>[2x]ATAQMQPDFWANQQAQFANEQNRLEQERVQQLQQQQAQQELFQQQLQKAQQDMMNMQLQQQNQHQNDLIALTNQYEKDQALLQQYDQRVQQLESEITTMDSTASKQLANKDEQLTALQDQLDVWERKYESLAKLYSQLRQEHLNLLPRFKKLQLKVNSAQESIQKKEQLEHKLKQKDLQMAELVKDRDRARLELERSINNAEADSAAATAAAETMTQDKMNPILDAILESGINTIQESVYNLDSPLSWSGPLTPPTFLLSLLESTSENATEFATSFNNLIVDGLAHGDQTEVIHCVSDFSTSMATLVTNSKAYAVTTLPQEQSDQILTLVKRCAREAQYFFEDLMSENLNQVGDEEKTDIVINANVDMQEKLQELSLAIEPLLNIQSVKSNKETNPHSELVATADKIVKSSEHLRVDVPKPLLSLALMIIDAVVALVK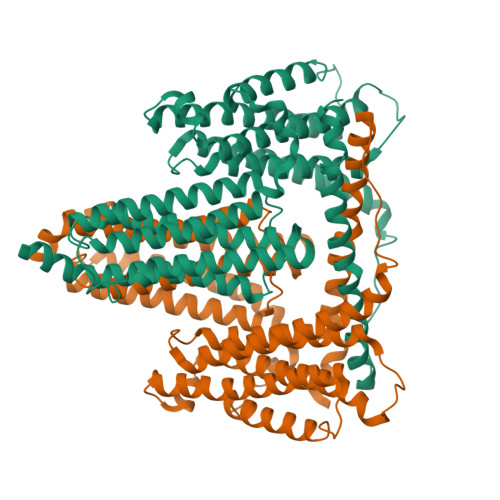AAIQCQNEIATTTSIPLNQFYLKNSRWTEGLISAAKAVAGATNVLITTASKLITSEDNENTSPEQFIVASKEVAASTIQLVAASRVKTSIHSKAQDKLEHCSKDVTDACRSLGNHVMGMIEDDHSTSQQQQPLDFTSEHTLKTAEMEQQVEILKLEQSLSNARKRLGEIRRHAYYNQDDD>[2x]ENYLDL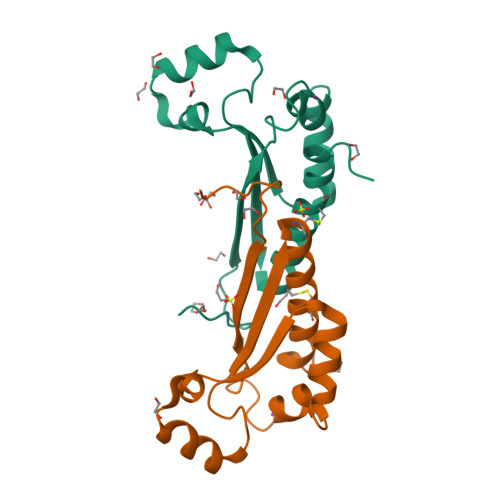FSHKNMKLKERVLIPVKQYPKFNFVGKILGPQGNTIKRLQEETGAKISVLGKGSMRDKAKEEELRKGGDPKYAHLNMDLHVFIEVFGPPCEAYALMAHAMCEVKKFLVPDMM> GFRASRSHSRREEHSGRNGLHHPSPDHFWPRFPDALRPFVPWDQLENEDSSVHISPRQKRDANSSIYKGKKCRMESCFDFTLCKKNGFKVYVYPQQKGEKIAESYQNILAAIEGSRFYTSDPSQACLFVLSLDTLDRDQLSPQYVHNLRSKVQSLHLWNNGRNHLIFNLYSGTWPDYTEDVGFDIGQAMLAKASISTENFRPNFDVSIPLFSKDHPRTGGERGFLKFNTIPPLRKYMLVFKGKRYLTGIGSDTRNALYHVHNGEDVVLLTTCKHGKDWQKHKDSRCDRDNTEYEKYDYREMLHNATFCLVPRGRRLGSFRFLEALQAACVPVMLSNGWELPFSEVINWNQAAVIGDERLLLQIPSTIRSIHQDKILALRQQTQFLWEAYFSSVEKIVLTTLEIIQDRIFKHIS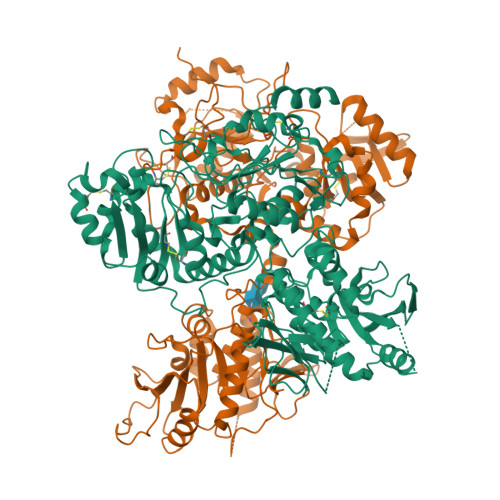RNSLIWNKHPGGLFVLPQYSSYLGDFPYYYANLGLKPPSKFTAVIHAVTPLVSQSQPVLKLLVAAAKSQYCAQIIVLWNCDKPLPAKHRWPATAVPVVVIEGESKVMSSRFLPYDNIITDAVLSLDEDTVLSTTEVDFAFTVWQSFPERIVGYPARSHFWDNSKERWGYTSKWTNDYSMVLTGAAIYHKYYHYLYSHYLPASLKNMVDQLANCEDILMNFLVSAVTKLPPIKVTQKKQYKETMMGQTSRASRWADPDHFAQRQSCMNTFASWFGYMPLIHSQMRLDPVLFKDQVSILRKKYRDIERL;> GWPHSIESSNDWNVEKRSIRDVPVVRLPADSPIPERGDLSCRMHTCFDVYRCGFNPKNKIKVYIYALKKYVDDFGVSVSNTISREYNELLMAISDSDYYTDDINRACLFVPSIDVLNQNTLRIKETAQAMAQLSRWDRGTNHLLFNMLPGGPPDYNTALDVPRDRALLAGGGFSTWTYRQGYDVSIPVYSPLSAEVDLPEKGPGPRQYFLLSSQVGLHPEYREDLEALQVKHGESVLVLDKCTNLSEGVLSVRKRCHKHQVFDYPQVLQEATFCVVLRGARLGQAVLSDVLQAGCVPVVIADSYILPFSEVLDWKRASVVVPEEKMSDVYSILQSIPQRQIEEMQRQARWFWEAYFQSIKAIALATLQIINDRIYPYAAISYEEWNDPPAVKWGSVSNPLFLPLIPPQSQGFTAIVLTYDRVESLFRVITEVSKVPSLSKLLVVWNNQNKNPPEDSLWPKIRVPLKVVRTAENKLSNRFFPYDEIETEAVLAIDDDIIMLTSDELQFGYEVWREFPDRLVGYPGRLHLWDHEMNKWKYESEWTNEVSMVLTGAAFYHKYFNYLYTYKMPGDIKNWVDAHMNCEDIAMNFLVANVTGKAVIKVTPRKKFKCPECTAIDGLSLDQTHMVERSECINKFASVFGTMPLKVVEHRADPVLYKDDFPEKLKSFPNIGSL>[2x]MTAKDIATEESKIRAYAQWMEI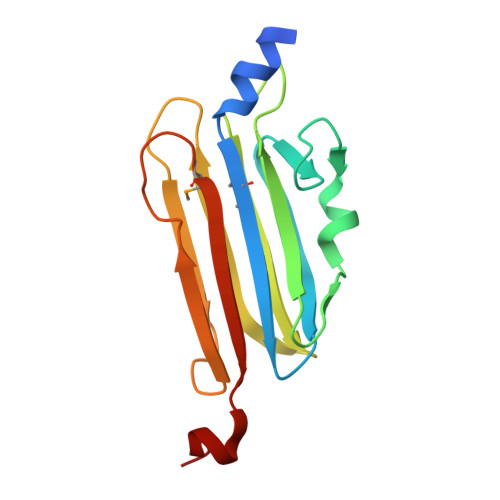TIFVVNSNFKVEGAYLRWGKFHVPGDKDKEISPSQINGTIIKDEDSYTIASCGRENASSGTEGGFSLYDGDKLVFEYYWDCPWSGSNSDELTVKDKENYTVIKKGGGSPSGAMGNIFITVVKKSLEHHHHHH>[2x]MILWRISAYADLSGTGGLRVSGAWHQAGRPVVYAATSPPGAMLEVLVHLEIDPEDFPTTMRLLRIE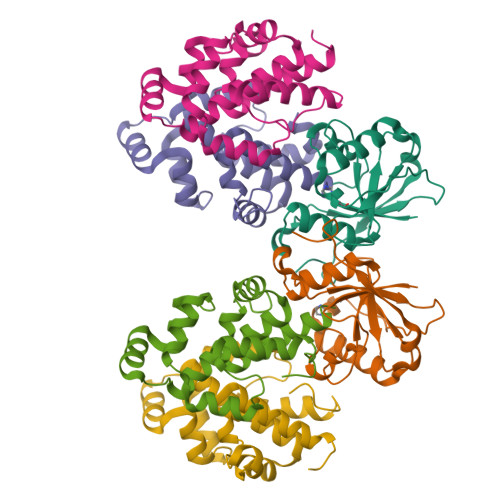LPDTVSQAQLPALQPGWSAQPELTRTLGNRFLDDCSALLLPVPSAIMPSTTNYLFNPRHPQAQSAKIQVEDFTPDSRLF;>MLAEVLRDNGYHEYRARLQALLDIPELASDFEIHTRITDGFAATWLVKLTERGVLTPVERDQIIPLRTLKSRIERDQPLTVDESDRLFRSAHITAMAEAVFGEAGKAKRWLSKPKERFSGLTPMQMLTTQQGTTQVEEMLLQIAEGYGL[4x]2-(1-((5-chloro-1H-pyrrolo[2,3-b]pyridine-3-carboxamido)methyl)-2-azabicyclo[2.1.1]hexan-2-yl)-N-methyl-4-(trifluoromethyl)thiazole-5-carboxamide | C20 H18 Cl F3 N6 O2 S | 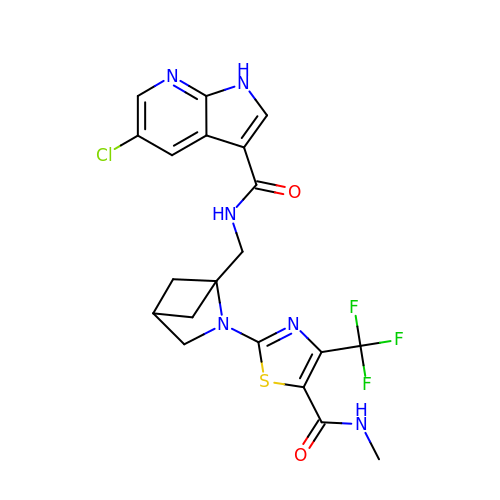JMSXCJHWSPPQRP-PJDKCZNOSA-N>MHHHHHHGSSYEKYKNAEKKFWHPMGSSAAPHRDKTLVIARGDGNYITDIDGQRMLDGVGGLWNVNIGHNRASVKAAIAAQLDELAYYQTFDGIAHPRVFDLAERLTGMFAQERMARVLFSSGGSDAVETALKMARQYWIASGEPGRTRFLSLRNGYHGVHMGGTSVGGNGVYHYNHGQLLAGCHLLDTPWLYRNPWDCRDPQALTAHCIRQLEEQIALLGAQTIAALIAEPVQGAGGVIVPPADYWPRLREVCDRHGILLIADEVVTGFGRSGCMLGSRGWGVAPDILCLAKGITAGYIPLGATLFNQRIADAIENGQGFSHMIMHGYTYSGHPTACAAALAVLDIVEAEDLPGNAAKVGAQLLEQLQPLVERYAVVGEVRGKGLMIALDLVSDKRTRQPLDPAAGQPSRIAD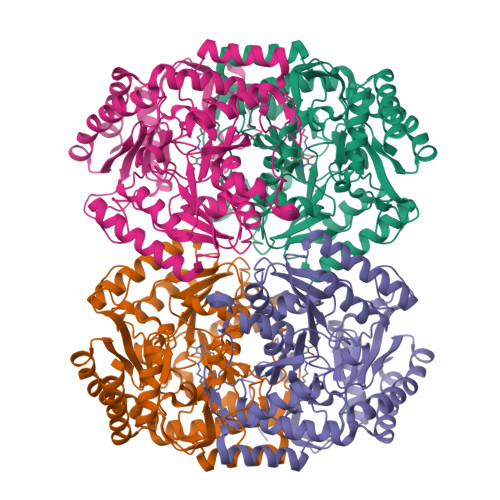EARRAGVLVRPIGNKIILSPPLTLTRDEAGLMVSALEAAFARCG[4x]> TWLPLNPIPLKDRVSMIFLQYGQIDVIDGAFVLIDKTGIRTHIPVGSVACIMLEPGTRVSHAAVRLAAQVGTLLVWVGEAGVRVYASGQPGGARSDKLLYQAKLALDE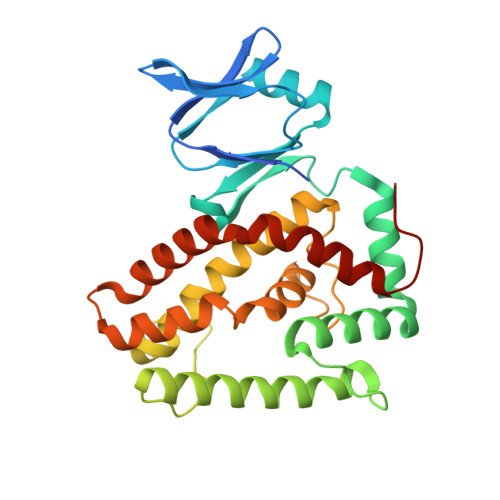DLRLKVVRKMFELRFGEPAPARRSVEQLRGIEGSRVRATYALLAKQYGVTWNGRRYDPKDWEKGDTINQCISAATSCLYGVTEAAILAAGYAPAIGFVHTGKPLSFVYDIADIIKFDTVVPKAFEIARRNPGEPDREVRLACRDIFRSSKTLAKLIPLIEDVLAAGEIQPPA> GGGGGGAMVEQYLLEAIVRDARDGITISDCSRPDNPLVFVNDAFTRMTGYDAEEVIGKNCRFLQRGDINLSAVHTIKIAMLTHEPCLVTLKNYRKDGTIFWNELSLTPIINKNGLITHYLGIQKDVSAQVILNQTLHEENHLLKSNKEMLEYLVNIDALTGLHNRRFLEDQLVIQWKLASRHINTITIFMIDIDYFKAFNDTYGHTAGDEALRTIAKTLNNCFMRGSDFVARYGGEEFTILAIGMTELQAHEYSTKLVQKIENLNIHHKGSPLGHLTISLGYSQANPQYHNDQNLVIEQADRALYSAKVEGKNRAVAYREQ

Here, we characterize a LOV-activated diguanylate cyclase (LadC) that offers precise temporal and spatial control of enzymatic activity with an exceptionally high dynamic range over four orders of magnitude. The blue-light sensor used in this system is a light-oxygen-voltage (LOV) domain, featuring a canonical flavin adduct upon blue light illumination. Here, we present a blue-light sensor coupled to a GGDEF effector domain that features exceptionally high fold changes of activation upon illumination. The name of the latter domain refers to a highly conserved sequence motif in the active site of GGDEF domains that enables GTP coordination and eventually diguanylate cyclase activity. To establish this pronounced activation, the enzyme exhibits a two-stage activation process in which its activity is inhibited in the dark by caging its effector domains and stimulated upon illumination by the formation of an extended coiled-coil.

The structure was solved by a combination of molecular replacement and single-wavelength anomalous diffraction (MR-SAD) phasing. The pyrophosphate was apparently copurified from the bacterial expression cultures, while FMN was added in excess during the purification process and Mg2+ was included as part of the purification buffers. Visualization of symmetry mates revealed a parallel dimeric assembly of MsLadC as the biological unit consistent with its in-solution behavior. Proteins, Interfaces, Structures and Assemblies (PISA) analysis supports this assembly with a large buried surface area between the two protomers (2785 Å2, ignoring ligand contacts) and high free energy of assembly dissociation (14.2 kcal/mol). Overall, the structure reveals a characteristic LOV-dimer interdomain interface, comprising the A′α helices and the core β sheet of the LOV domain. The structure reveals a tight interaction of the LOV domains with their C-terminally linked GGDEF domains. In addition, the inhibitory interface is formed between the surfaces of the LOV and GGDEF domains. For example, Asp44# (hashtag denotes the adjacent protomer) from the LOV’s Cα-Dα loop forms a salt bridge with Arg174 from the GGDEF’s α0 helix, and Glu77 from the LOV’s Fα-Gβ loop interacts with Gln242 from the GGDEF’s α3 helix. The buried surface area of the inhibitory interface in the dimeric assembly amounts to 3073 Å2, as calculated using PISA. This interaction interface, together with interactions within the linker region, explains the inactive, “switched off,” dark state. S7C, the MsLadC dark-state crystal structure superposes well with the MsLadC dark-state SAXS envelope (χ2 of 0.999), confirming the crystallographic assembly as a functionally relevant inhibited state in solution.>[2x]MSKNK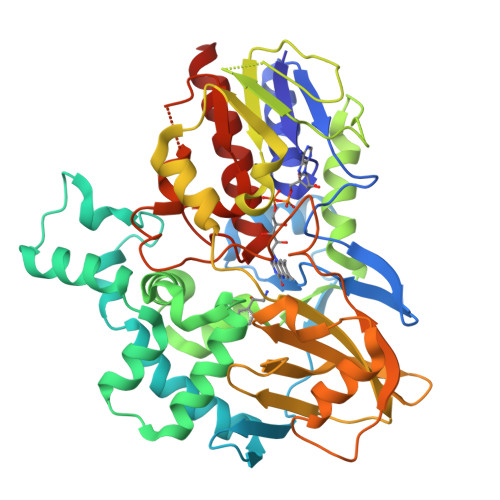VVIIGAGFAGLVAARELQTAGIEYEILEAKDRIGGRAWTEERMGRPLELGATWVHWFQAHTWTEIMRYGQRTEITASPSGNDAHWVTDGKVVKGTEDDLDEKLTAAMGVTYEGSEEYFPNPHDPLWVLSDDFDGPAEVRERFLSDDQTNAIDLVKEAGFDQETIDLVDAFWCAGYIGDPYTGSALMAKQWGALSDNRYRVMEDITLKWKLNNGMRSLYDGIAGDLNTDIRLNTPVAKVEHHDNGATVTTESGEVIEASAVICTVPVGALSNIEFSPALPDAVQSVIDDKWNSQGAKIWIKIKGHHRFLGYAPKPAKMSVVRSEYFMDDDTTILVGFGYDNTNIDLNSIEDAQAVINQWRDDLEVVDTTGHNWVADKWAGQAWGTLRKGQFTQGWSLFDDIDSQLFFAGSDYAYGWRGVCVDGALEKGMTTARQVINSMRETKEQ N-[(1S)-2-[(2-amino-5-quinolyl)methylamino]-1-benzyl-2-oxo-ethyl]-4-hydroxy-2-oxo-1H-quinoline-6-carboxamide | C29 H25 N5 O4 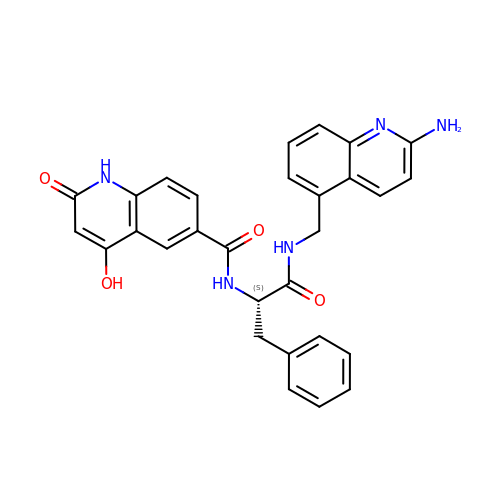| WHPQJMIXRFKMJB-DEOSSOPVSA-N> VQRVEGKLRASVEKGDYYEAHQMYRTLFFRYMSQSKHTEARELMYSGALLFFSHGQQNSAADLSMLVLESLEKAEVEVADELLENLAKVFSLMDPNSPERVTFVSRALKWS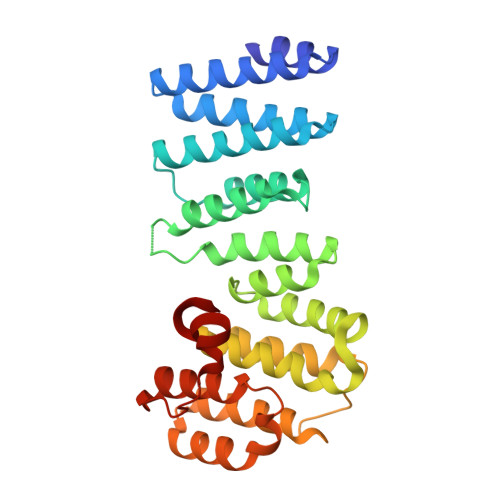SGGSGKLGHPRLHQLLALTLWKEQNYCESRYHFLHSADGEGCANMLVEYSTSRGFRSEVDMFVAQAVLQFLCLKNKSSASVVFTTYTQKHPSIEDGPPFVEPLLNFIWFLLLAVDGGKLTVFTVLCEQYQPSLRRDPMYNEYLDRIGQLFFGVPPKQTSSYGGLLGNLLTSL> GSHMTNWLRVYYYEDTISTIKDIAVEEDLSSTPLLKD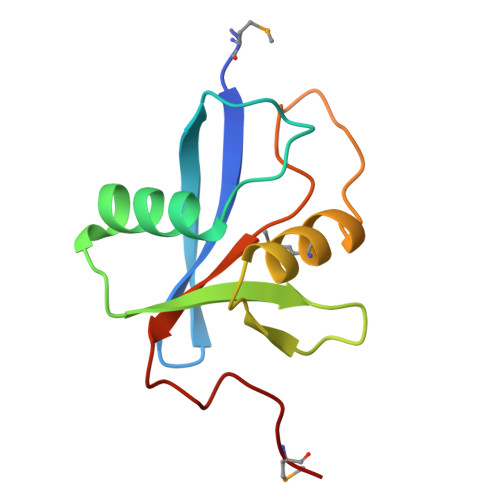LLELTRREFQREDIALNYRDAEGDLVRLLSDEDVALMVRQARGLPSQKRLFPWKLHITQKDNYRVYNTMP> MHHHHHHKLITLLLRSSKSEDLRLSIPVDFTVKDLIKRYCTEVKISFHERIRLEFEGEWLDPNDQVQSTELEDEDQVSV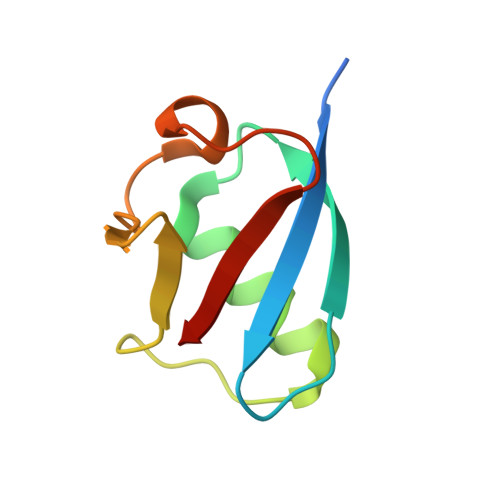VLD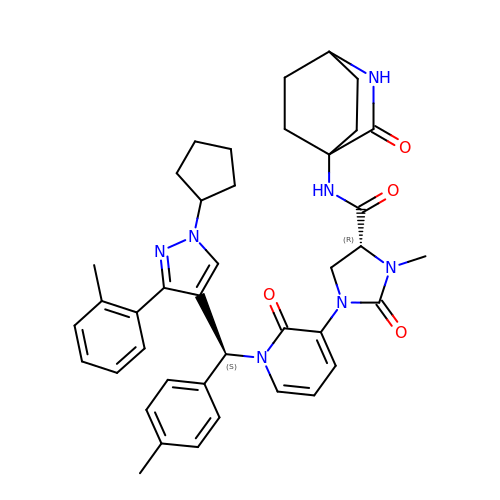(4R)-1-[1-[(S)-[1-cyclopentyl-3-(2-methylphenyl)pyrazol-4-yl]-(4-methylphenyl)methyl]-2-oxidanylidene-pyridin-3-yl]-3-methyl-2-oxidanylidene-N-(3-oxidanylidene-2-azabicyclo[2.2.2]octan-4-yl)imidazolidine-4-carboxamide | C40 H45 N7 O4 | GUMPNBZZBQKOPS-KFTXPEDNSA-N5'-{[(3S)-3-amino-3-carboxypropyl][2-(hexylamino)ethyl]amino}-5'-deoxyadenosine 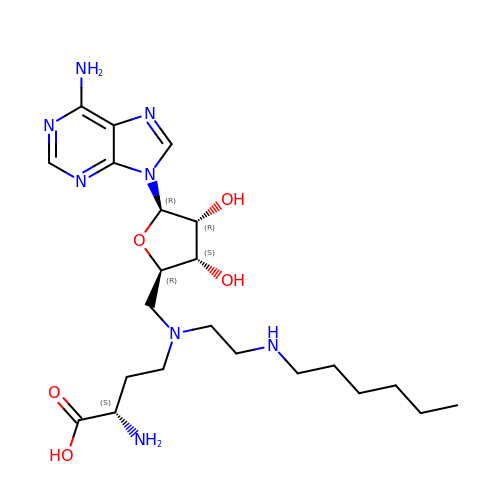| C22 H38 N8 O5 | XWQXPIOHEBRBJA-UQEZQTQMSA-N> MSLDEDKTNDSAFHARLIAEVLEAYPDKARKRRQKHLNVAGQAEAEAQDAGEEGVMLSECDVKSNVKSVPGVMTIRGCAYAGSKGVVWGPVKDMVHISHGPVGCGQYSWSQRRNYYIGNTGVDSFVTMQFTSDFQEKDIVFGGDKKLEKIIDEIDELFPLAKGISVQSECPIGLIGDDIEAVSRKKKKEIGKTIVPVRCEGFRGVSQSLGHHIANDAIRDWVFDGEDKHAAFETTPYDVNVIGDYNIGGDAWSSRILLEEMGLRVVGNWSGDATLAEIERAPKAKLNLIHCYRSMNYICRHMEEKYNIPWTEYNFFGPSQIAASLRKIAALFDEKIQEGAERVIAKYQPLVDAVIEKFRPRLAGKKVMLYVGGLRPRHVVNAYNDLGMEIVGTGYEFGHNDDYQRTGHYVREGTLIYDDVTGYELEKFIEGIRPDLVGSGIKEKYPVQKMGIPFRQMHSWDYSGPYHGYDGFAIFARDMDLAINNPVWSMFKAPWKN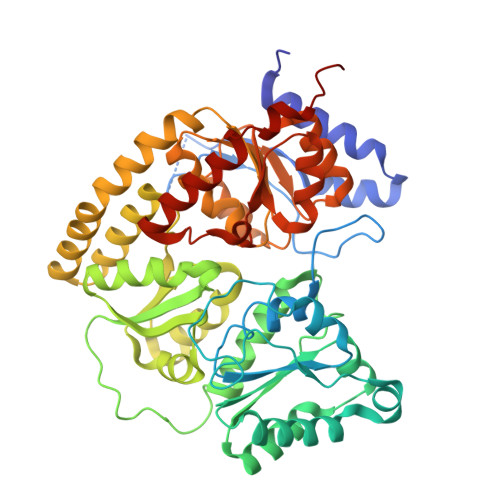AA HDACs form 2 major families: Zn++-dependent HDACs and NAD+-dependent HDACs, also termed sirtuins (SIRTs). SIRT2 has deacylation activities in addition to deacetylation, including demyristoylation, and several SIRT2 inhibitors are acyl group selective, blocking deacetylation but not demyristoylation. The structures consist of 2 domains: an upper Zn++-binding domain and a lower catalytic domain with a Rossmann fold. The 2 domains behave as a clamshell, accommodating varying acyl-Lys modifications within a flexible pocket between the 2 clamshell domains.

We produced crystals of FLS-359 bound to SIRT2 that diffracted to 1.8 Å resolution and determined the structure of the complex. FLS-359 bound SIRT2 between its Zn++-binding domain and the catalytic Rossmann fold domain, in the EC pocket where other small-molecule ligands have been localized. The binding interactions of FLS-359 with SIRT2 include π-π interactions with residues F119, F190, and Y139. Water residue 566 bridges FLS-359 and SIRT2 with one hydrogen bond to the thiazole of FLS-359 and another hydrogen bond to the backbone carbonyl of residue F96. A multi-body water network in the peptide channel connects, via a hydrogen bond network, the dimethyl imidazole of FLS-359 to E116 through water residue 371 and to the side chain of R97 through water residues 371, 165, and 652. These water-mediated hydrogen bonds could be key interactions that drive binding affinity to SIRT2 in the hydrophobic EC site. NAD+ binding is not predicted to be affected by FLS-359 binding. In contrast, the FLS-359 dimethylimidazole moiety resides in the same location as the peptidic acetyl group, but computational superpositioning predicts that the pocket can accommodate both FLS-359 and the peptide. Modeling predicts that SIRT2 can accommodate both an acetyl group and FLS-359, whereas the binding of a myristoyl group excludes FLS-359. In sum, enzyme thermal denaturation and kinetics studies, as well as co-crystal structure determination, argue that FLS-359 binds selectively to SIRT2 and induces an allosteric rearrangement of the active site, reducing the rate of deacetylation.

>[2x]ERLLDELTLEGVARYMQSERCRRVICLVGAGISTSAGIPDFRSPSTGLYDNLEKYHLPYPEAIFEISYFKKHPEPFFALAKELYPGQFKPTICHYFMRLLKDKGLLLRCYTQNIDTLERIAGLEQEDLVEAHGTFYTSHCVSASCRHEYPLSWMKEKIFSEVTPKCEDCQSLVKPDIVFFGESLPARFFSCMQSDFLKVDLLLVMGTSLQVQPFASLISKAPLSTPRLLINKEKAGQSDPFLGMIMGLGGGMDFDSKKAYRDVAWLGECDQGCLALAELLGWKKELEDLVRREHASIDAQS> MDQKASYFINEKLFTEVKPVLFTDLIHHLKIGPSMAKKLMFDYYKQTTNAKYNCVVICCYKDQTIKIIHDLSNIPQQDSIIDCFIYAFNPMDSFIPYYDIIDQKDCLTIKNSYELKVSESSKIIERTKTLEEKSKPLVRPTARSKTTPEETTGRKSKSKDMGLRSTALLAKMKKDRDDKETSRQNELRKRKEENLQKINKQNPEREAQMKELNNLFVEDDLDTEEVNGGSKPNSPKETDSNDKDKNNDDLEDLLETTAEDSLMDVPKIQQTKPSETEHSKEPKSEEEPS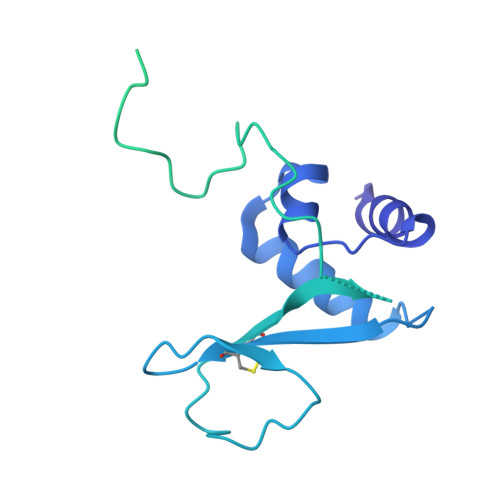SFIDEDGYIVTKRPATSTPPRKPSPVVKRALSSSKKQETPSSNKRLKKQGTLESFFKRKAK>[4x]MKQTSLEVKEFALNLISQFEPENQPLGFWIFDTEGVEKAVERWKKNMPTVRPCFAVKCNPEPHLVKLLGELGCGFDCASLNEIKEVLDLGFNPEDITYSQTFKPYNQLIEASHLGINHTIVDSIDEVQKIAKYAPKMGI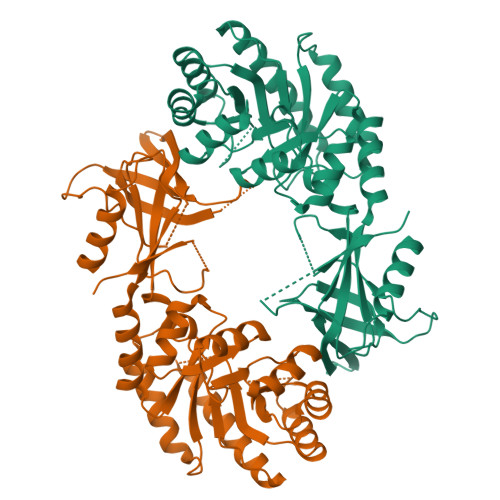MIRIMENDTSAGHVFGEKFGLHDDEVEIVLKEIKDKGLNLDGVHFHVGSDSHNSEVFTKALTKARNTVTLAEQFGMKPYLIDIGGGFSQVAPFEEFAATIEKTIKELEFPERTRFIAEPGRYMASNAFHLVSSLHGKRVRIQNGKKQIEYTSGDGLHGSFGCCIWFEKQKSCECITQKVNENTKMYESIIYGPSCNGSDKVATQELPEMEPGKDWLLFPNMGAYTISMATNFNGFEERNHVIYTLPLKSTKIIQIP>MSSSGTPDLPVLLTDLKIQYTKIFINNEWHDSVSGKKFPVFNPATEEELCQVEEGDKEDVDKAVKAARQAFQIGSPWRTMDASERGRLLYKLADLIERDRLLLATMESMNGGKLYSNAYLSDLAGCIKTLRYCAGWADKIQGRTIPIDGNFFTYTRHEPIGVCGQIIPWNFPLVMLIWKIGPALSCGNTVVVKPAEQTPLTALHVASLIKEAGFPPGVVNIVPGYGPTAGAAISSHMDIDKVAFTGSTEVGKLIKEAAGKSNLKRVTLELGGKSPCIVLADADLDNAVEFAHHGVFYHQGQCCIAASRIFVEESIYDEFVRRSVERAKKYILGNPLTPGVTQGPQIDKEQYDKILDLIESGKKEGAKLECGGGPWGNKGYFVQPTVFSNVTDEMRIAKEEIFGPVQQIMKFKSLDDVIKRANNTFYGLSAGVFTKDIDKAITISSALQAGTVWVNCYGVVSAQCPFGGFKMSGNGRELGEYGFHEYTEVKTVTVKISQKNS[4x]

Here we report the use of “Build and Retrieve” to define the composition of a raw human brain microsomal lysate. From this sample, we simultaneously identify and solve cryo-EM structures of five different brain enzymes whose functions affect neurotransmitter recycling, iron metabolism, glycolysis, axonal development, energy homeostasis, and retinoic acid biosynthesis. Collectively, the BaR approach was then used to reveal enzyme identities and solve cryo-EM structures of these brain enzymes with resolutions ranging between 2.69 and 3.40 Å. These enzymes were identified as glutamine synthetase (GS), ferritin (FT), dihydropyrimidinase-related protein 2 (DPYSL2), glyceraldehyde 3-phosphate dehydrogenase (GAPDH), and retinaldehyde dehydrogenase 1 (ALDH1A1). Interestingly, malfunction of these important proteins has been directly linked to several neurodegenerative disorders, such as Alzheimer’s, Huntington’s, and Parkinson’s diseases.

The ALDH1A1 enzyme plays a primary role in the biosynthesis of retinoic acid, an important signaling molecule that specifically interacts with the retinoic acid receptor. Subsequently, we were able to identify this protein as the ALDH1A1 enzyme and resolve its structure to a resolution of 3.40 Å. ALDH1A1 assembles as a tetramer in oligomerization. Each subunit of ALDH1A1 can be divided into cofactor-binding (green), catalytic (blue), and oligomerization (orange) domains. Presumably, residues I166, P168, W169, K193, E196, Q197, P227, F244, A231, S234, V250, S247, C303, Q350, K353, E400, and F402 are engaged in NAD+ binding. In our cryo-EM structure, we did not observe bound NAD+ in our structure. The catalytic site of ALDH1A1 is surrounded by residues L114, S121, K128, T129, W178, I304, V459, V460, S461, and A462. Two missense mutations, A151S and I157T, have been identified for the human ALDH1A2 enzyme, where these two mutations are strongly associated with congenital heart disease. The corresponding residues in ALDH1A1 are A134 and I140. These two residues are located at the subunit–subunit interface and are probably critical for the tetrameric oligomerization of this enzyme.>[4x]SCVRDNSLVRDISQMPQSSYGIEGLSHITVAGALNHGMKEVEVWLQT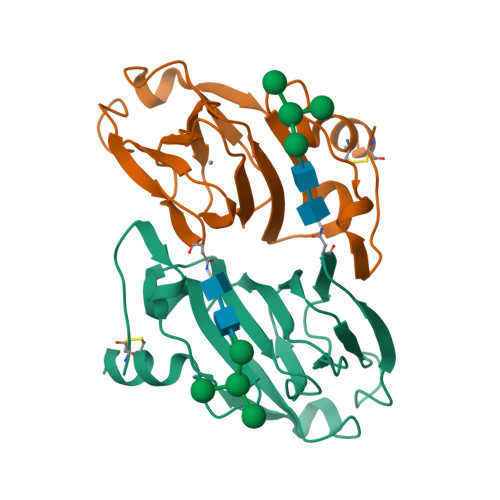ISPGQRTPIHRHSCEEVFTVLKGKGTLLMGSSSLKYPGQPQEIPFFQNTTFSIPVNDPHQVWNSDEHEDLQVLVIISRPPAKIFLYDDWSMPHTAAVLKFPFVWDEDCFEAAKEQL(5S)-2-amino-5-[(1R)-1-(1H-indol-3-yl)ethyl]-1,3-oxazol-4(5H)-one | C13 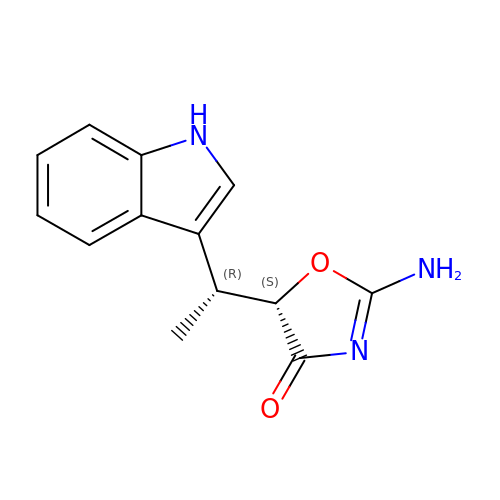H13 N3 O2 | JMQXZRUQJGJVSC-HQJQHLMTSA-N>[2x]MKKKTASLRMKTLAAGAAVAAALSMGAVTDLPGAKWLHPAAAQAAETVFKQNHAASGFLAGRYDAQAMSPTMFNWSRESRFTSTADGALKWEKNVPATP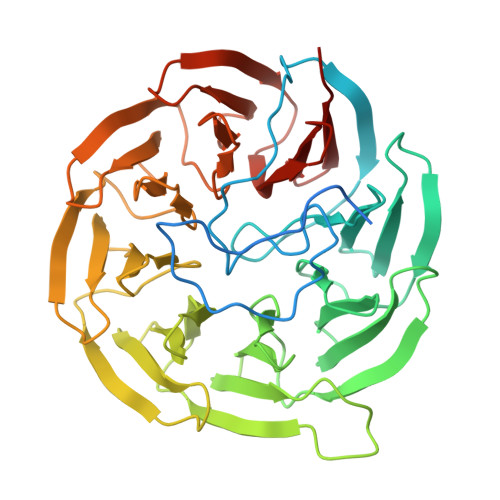QNGAGAAVDGDGTVFIQSKDGKLTAYHPDGTVKWVTENLGTTYTLTPVLGTNGVIYLPSHDKKLYFIDKETGNILWSVPLSGAPSSDAAIGPDGTLYVSTLDNYIYAIKPTSPSTGTQKWKFKTNGVVGSAPVLASNGTLYTATYNNIFYAINSGTGQVKWSKTTSNGFKGYPVIDRDGTVYAGNQDGNLYAYTSTGAVKWTFPLNGFSSSSLAIDHNGNVYIGSGSGELFSISKTGNMNWSFYTDGPVRTAPLIDADGNVYFGSDDKNVYAVDADGNEKWRYQTDSNVISSPVLAEDGTLYVGTYTKLLAFGAKK>VEYRNWSKPQCQITGFAPFSKDNSIRLSAGGDIWVTREPYVSCDPGKCYQFALGQGTTLDNKHSNDTVHDRIPHRTLLMNELGVPFHLGTRQVCIAWSSSSCHDGKAWLHVCITGDDKNATASFIYDGRLVDSIGSWSQNILRTQESECVCINGTCTVVMTDGSASGRADTRILFIEEGKIVHISPLSGSAQHIEECSCYPRYPGVRCICRDNWKGSNRPVVDINMEDYSIDSSYVCSGLVGDTPRNDDSSSNSNCRNPNNERGTQGVKGWAFDNGNDLWMGRTISKESRSGYETFKVIGGWS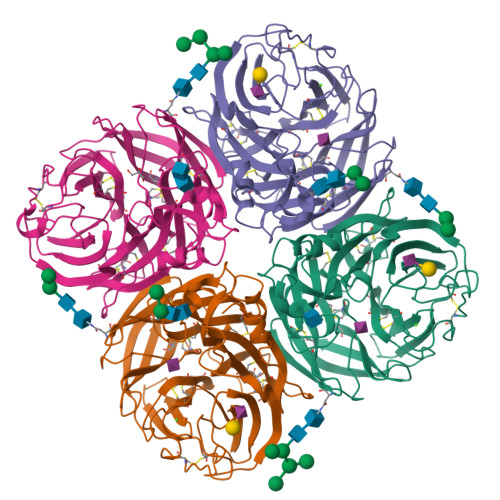TPNSKSQVNRQVIVDNNNWSGDSGIFSVEGKSCINRCFYVELIRGRPQETRVWWTSNSIVVFCGTSGTYGTGSWPDGANINFMPI[4x]>MQALTTYKCIEKGIVVWLTGLPGSGKTTIATRLADLLQKEGYRVEVLDGDWARTTVSEGAGFTREERLRHLKRIAWIARL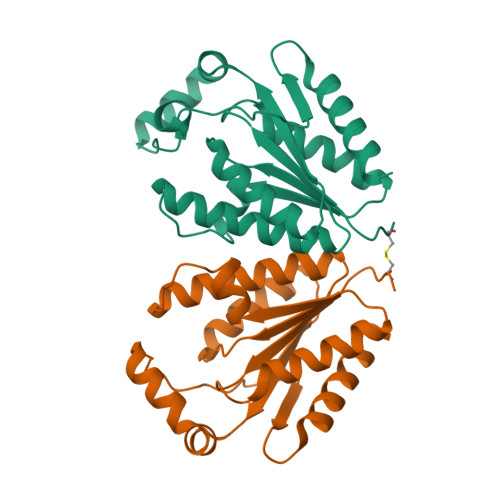LARNGVIVICSFVSPYKQARNMVRRIVEEEGIPFLEIYVKASLEEVIRRDPKGLYKKALKGELENFTGITDPYEPPENPQLVLDTESNTIEHNVSYLYSLVKAVIE[2x]> RNAEFKVSKNSTSFKNPRRLEIKDGRSLFLRNRGKIHSGVLSSIES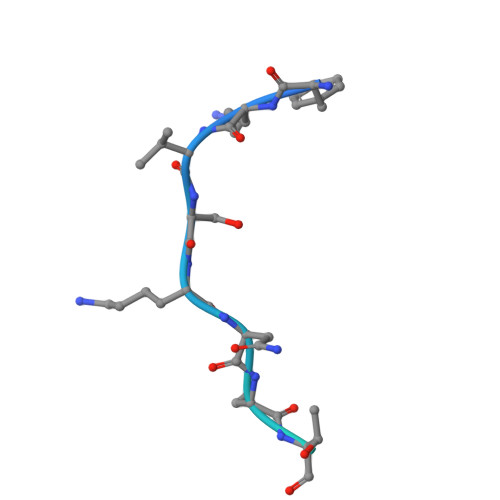DL> TSVPSSPLDYAIFSKGALNTNKNLTVENGSVYSGGDLTIDGGAVFNIDNLISKGEMVINQDSDSRCRDNNIVVRNIIYVEKSLKANRISPRSTNIDAKTIYVGQEMQLYGAGSYKFVQLFSDSNVKLAGPGVNMEVSTLASIRGTLEVIDGATVTLKSNSAVYCNSLVVRNGSRLI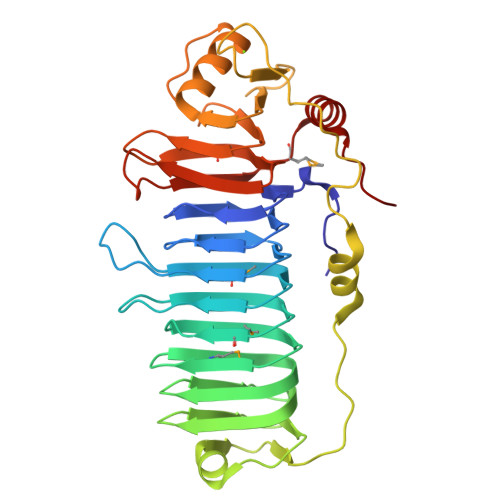LENGAKLYLATTPDASTIISIQNNGGTISYSSSFSYPSPPAEIDEIRNRDYTSGLLTTPLPADSVGSNQLGSTADTSQTPPQIVIYGESYINDNEARIEISARLGSPIVDFSTLQLHLISRGNITFVGGGLTIMNGSIISLGSTFNINATGNPYAGLTLKYQMPSPPIQQDIESNTGIQPSQ> STPAITLENPDIKYPLRLIDKEVVNHDTRRFRFALPSPEHILGLPVGQHIYLSARIDGNLVIRPYTPVSSDDDKGFVDLVIKVYFKDTHPKFPAGGKMSQYLESMKIGDTIEFRGPNGLLVYQGKGKFAIRPDKKSSPVIKTVKSVGMIAGGTGITPMLQVIRAIMKDPDDHTVCHLLFANQTEKDILLRPELEELRNEHSARFKLWYTVDRAPEAWDYSQGFVNEEMIRDHLPPPEEEPLVLMCGPPPMIQYACLPNLERVGHPKERCFAF

NADH-cytochrome b5 reductase (b5R; EC 1.6.2.2) is a flavoprotein containing one FAD molecule. A single-spanning transmembrane helix anchors the protein on the inner surface of the endoplasmic reticulum membrane. b5R mediates electron transfer from NADH to cytochrome b5 (b5). Flavin compounds such as flavin adenine dinucleotide (FAD), flavin mononucleotide (FMN) and riboflavin (vitamin B2) are utilized as cofactors of proteins for various oxidoreductive processes. The isoalloxazine ring is a redox center common to all of these compounds.

The valence electronic structures of FAD as well as the protein environment are experimentally determined and analyzed in order to investigate the properties of FAD in b5R. The most unexpected feature of FAD in b5R is the lone pair distributions around the N5 atom. On the other hand, we have to worry that the electronic distribution around N5 is an experimental and/or analytical artifact. However, we believe that the result is relevant for two reasons as follows. First, the radiation damages could be suppressed by the collection of data at low accumulated doses (1.8 × 105 Gy for the first data set and 0.9 × 105 Gy for the second data set) at 40 K. The values were smaller than the Henderson limit of 2.0 × 107 Gy applied to ordinal measurements around 100 K by more than two orders of magnitude. The second reason is that the valence electrons were clearly observed for both Data I and II, even in the residual maps of the ISAM refinements as well as the deformation maps of the MAM refinements. These multiple results enhance the validity of this study.> MEVNEKAPAQARPTVFRWTGGGKEVYLSGSFNNWSKLPLTRSQNNFVAILDLPEGEHQYKFFVDGQWTHDPSEPIVTSQLGTVNNIIQVKKTDFEVFDALMVDSQKCSDVSELSSSPPGPYHQEPYISKPEERFKAPPILPPHLLQVILNKDTGISCDPALLP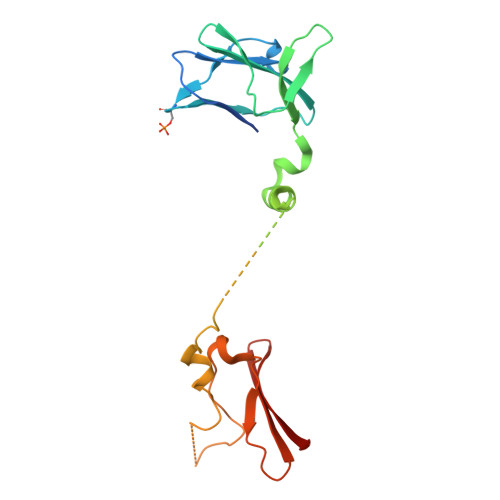EPNHVMLNHLYALSIKDGVMVLSATHRYKKKYVTTLLYKPI>MREVKLVTFDVWNTLLDLNIMLDEFSHQLAKISGLHIKDVANAVIEVRNEIKKMRAQASEDPRKVLTGSQEALAGKLKVDVELVKRATARAILNVDESLVLEGTKEALQFVKERGLKTAVIGNVMFWPGSYTRLLLERFGLMEFIDKTFFADEVLSYKPRKEMFEKVLNSFE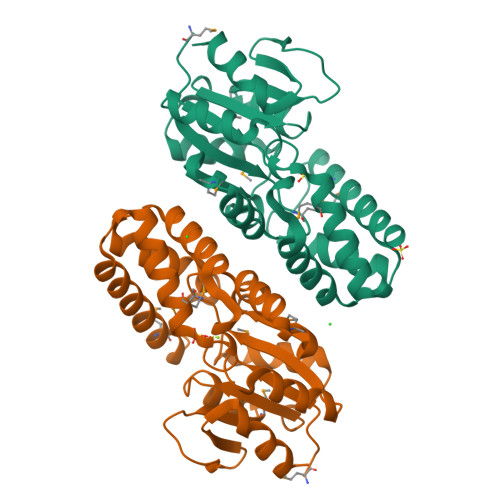VKPEESLHIGDTYAEDYQGARKVGMWAVWINQEGDKVRKLEERGFEIPSIANLKDVIELISKT[2x]>GPGSMAETLTEVTRQAAVVERRGNVALITIDRPDARNAVNGAVSTAVGDALEEAQRDPEVWAVVITGAGDKSFCAGADLKAISRGENLYHAEHPEWGFAGYVHHFIDKPTIAAVNGTALGGGSELALASDLVIACESASFGLPEVKRGLIAGAGGVFRIVEQLPRKVALELVLTGEPMTASDALRWGLINEVVPDGTVVEAALALAER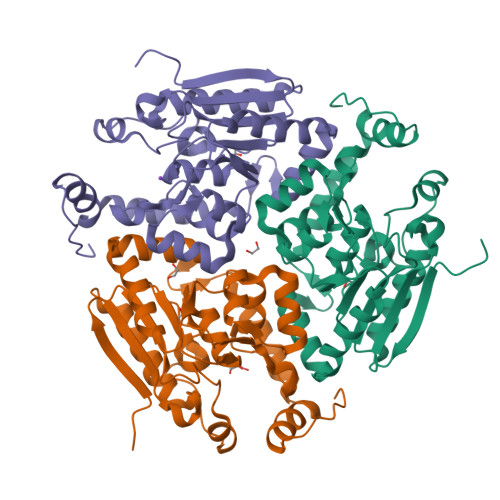ITCNAPLSVQASKRVAYGADDGIIGAEEPKWERTIREFTELLKSEDAKEGPLAFAEKRQPVWKAR[3x]> MRNKIFISHATPDDNDFTRWLALKLIGLGYEVWCDILFLDKGVDFWSNIEKVIREDTCKFLLVSSSYSNQREGVLKELAVAAKVKKQLKDDKFIIPLAIDEQLSYDDINIDIVRLNAIDFKMSWARGLKDILEAFEKQKVPKEVADASKSNLLYQQIFLHDKSVIEKEEIYDSNWLSI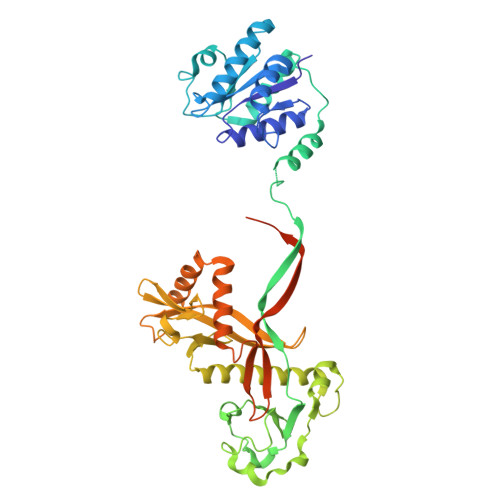LSFPEELRFHEYNWMLPKRFDVRELTFPAVRYKNYLCTFAWAYDFTYHLPKTETYHKSKTIRIPTEEILSGSYDSNFIRNAECKRLIVQLLNKAFELRMKDKEVQEYEMSNKTAYWLEKGKLEKDKFEKTMLVGKQKDKNWHFAISGASKLYPFPVLMISSHIFFTADGKKLIDSSSVQHSSRRRQGKNWWNNTWRTKLLAFIKYLSDDDTSFYLEMGSEEKVFVSNEPVKFKGNVSYNIPEKNTLEEEAELSGFNQGEDIEELEELIENLEAE> GDERFYAEHLMPTLQGLLDPESAHRLAVRFTSLGLLPRARFQDSDMLEVRVLGHKFRNPVGIAAGFDKHGEAVDGLYKMGFGFVEIGSVTPKPQEGNPRPRVFRLPEDQAVINRYGFNSHGLSVVEHRLRARQQKQAKLTEDGLPLGVNLGKNKTSVDAAEDYAEGVRVLGPLADYLVVNVSSPNTAGLRSLQGKAELRRLLTKVLQERDGLRRVHRPAV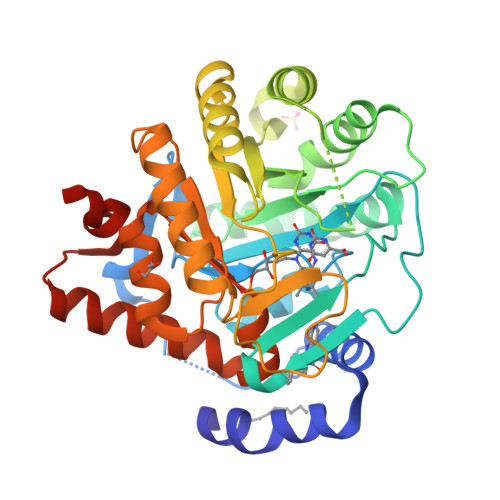LVKIAPDLTSQDKEDIASVVKELGIDGLIVTNTTVSRPAGLQGALRSETGGLSGKPLRDLSTQTIREMYALTQGRVPIIGVGGVSSGQDALEKIRAGASLVQLYTALTFWGPPVVGKVKRELEALLKEQGFGGVTDAIGADHRRLEAGHHHHHH> TNTDSFTFSKFKPNQPNLKKQGDATVTSSGTLQLTKVDKNGVPDPKSLGRALYASPINIWDSKTGVVASFATSFRFTIYAPNIATIADGLAFFLAPVSSPPKAGAGFLGLFDSAVFNSSYQTVAVEFDTYENTVFLDPPDTHIGIDVNSIKSIKTVKWDLANGEAAKVLITYDSSAKLLVAALVYPSSKTSFILSDVVDLKSVLPEWVSIGFSAATGASSGYIET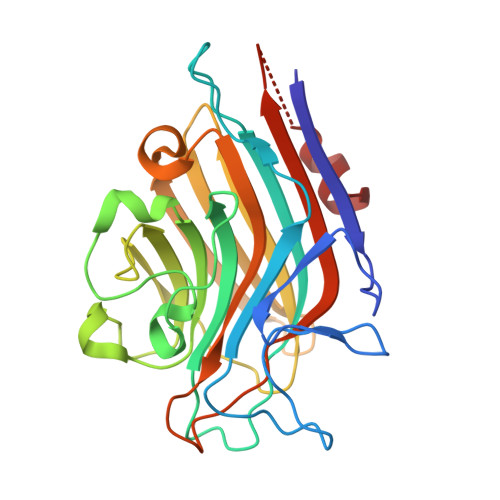HDVFSWSFASKLSFXXXXXXLDLASFLVAN> MDKINLVCGSLLHNIGKIIYRGTSERAKHSKLGGDFIKSFEQFRNTELTDCIRYHHAQEITSVKSNKEKNSLFYITYIADNISSGMDRRKDLEEGAEGFNWDKKVALGSVFNVLNEKEKGRQNYSYPFVARTRIKEEPLNFPTATQNQYTTSYYDGLITDMKTILQRLKPDKEHINSLLQMMESLWSYVPSSTDKNQLVDISLYDHSRTTAAIASAIYDYFQAENITDYQKELFDYNATEFYDKNAFLMMNFDMSGVQNFIYNISGSKALKSLRARSFYLDMLLEYISDNLLEKLELSRANILYVGGGHAYLLLANTNKTKAILSDFEHDLKTWFLDKFKIDLYVAMAYTEVSANDLMNHNGHYRDIYRRLSQKTSAKKANRYTAEEILNLNHQGTENARECRECKRSDLLIEEDDICEICDSLQKVSRDLTRENIFVIANEGVLDMPFGKKMSALSYSQADKLKKSNAEVQIYAKNISEIGQNLMTRIDMGDYTYRSDFHEMLEEVEVGINRLGVLRADVDNLGQAFINGIPDDYLSISRTATFSRAMSRFFKNYLNQLLAEKSYKINVIYAGGDDLFMIGAWQDILDFSIVLKQKFADFTQNKLSISAGIGMFREKYPVARMASLTGDLEDAAKDYKPDERAVQATKNAVTLFDATNVFSWDTLENDIFVKLDAITKNFEKLDETGKAFIYRLIDLLRGVNENQQINIARLAYTLSRMEEKIGKTFAQELYNWANADRKTLIMALEIYILKTRE;> MKIIKLYFESPVHFGEKRLSESKITFSADTLFSALMIEAVGLGKEDEFYQLASNNLVKFSDAFPFIDQYYYIPKPMFNLKLEKEDENPSKAFKKLLYVPIDSLEDYLSGGLDAYFERESFNLGKLALSEKVQQHDFKDSEPYNVGTFTFKENTGLYVLIEQTHPLLEELLENLQYSGIGGKRNSGYGKFKFEILEDSDIEDLFSAKGNRKILLSGALPKDAELEQALKNASYLLERRGGFVQSDTYATNLVKKQDLYVFKSGSTFENSFDGDIYQVGKKGNHPVYKYAKSFFLEVSV;>TELKIGNEKVNSTNFGDFAEKAIRGINHKPFVNSKGGEQKITTSKIRGILELVNKVYNRVINTNDVELSENILADIAYIKVKIAYESGREPVVKDFIQRTAFTAAITDVMNQRTRESFLLFARYVESLIAYFKFYGGKD[3x];>MKLVIEGTIVLKTGMHIGGSSDFSAIGAVASPVVRDTLTRLPLIPGSSLKGKMRYLLAKELNNGILLNEPNNDQDEILRLFGSSEKDKIRRARLKFNDIKLSNLAELETFNVSSTEVKFENTINRKTAVANPRQIERVIAGSKFDFEIFYNLDDIKEVEKDFENIKQGFDLLEFDYLGGHGTRGSGRIAFENLSVITAVGNFEKINTLNEILGA[4x];> MKKTYRVTLTALGPIFIGGGEKLKKYEYIFDKQKKVAHMIDHTKFTKYLLEK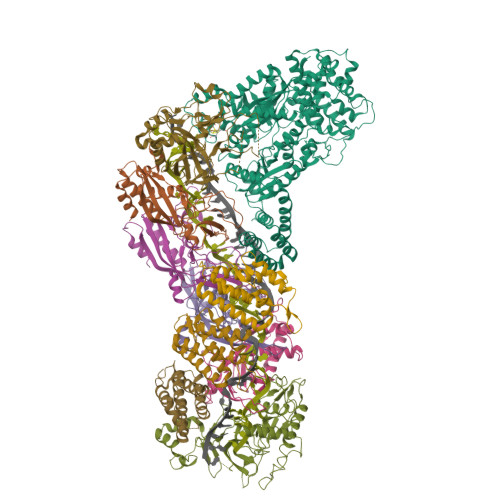NLLDDFTSRVNSHFDLYDYLVNKKGIVFMPLVKYSVPVAQFRTEVKNRFGKPISSPPMNDLNTFVKDAFGRPYIPGSSLKGALRTAILNDLKEDTKENEVFAHLQVSDSETIDLENLKVYQKVDYSKTAKPLPLYRECLKPNTEITFTVSFDDEYLTLKKIQNALHKTYQHYYIKWLKGGKVGETLIKGVYDSHADELKKNTFALDQPSQNQGEIIYIGGGAGFVSKTLHYKSKNRDQARNDSFDILKQLFRTTYSKMRSVPDNVPVALKLAVETKTFNGRVTGKHYLEMGKARIKLEEL>[2x]AIDPALPEYQKASGVSGNLSSVGSDTLANLMTMWAEEYKRLYPNVNIQIQAAGSSTAPPALTEGTANLGPMSRKMKDVELQAFE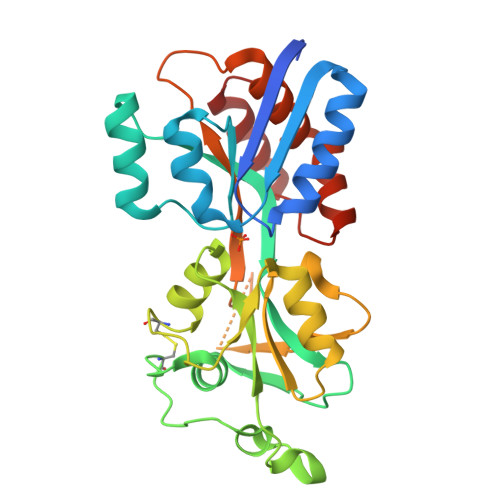QKYGYKPTAVPVAVDALAIFVHKDNPIKGLTMQQVDAIFSATRLCGSKQDVKTWGDLGLTGDWAKKPVQLFGRNSVSGTYGYFKEEALCKGDFRPNVNEQPGSASVVQSVSQSLNGIGYSGIGYKTASVKTVALAKKEGAAFVEDNEQNALNGTYPLSRFLYVYVNKAPNKPLDPLEAQFLKLVLSKTGQQVVVKDGYIPLPAKVAEKAIKELGL>[2x]GAMAKVQVNNVVVLDNPSP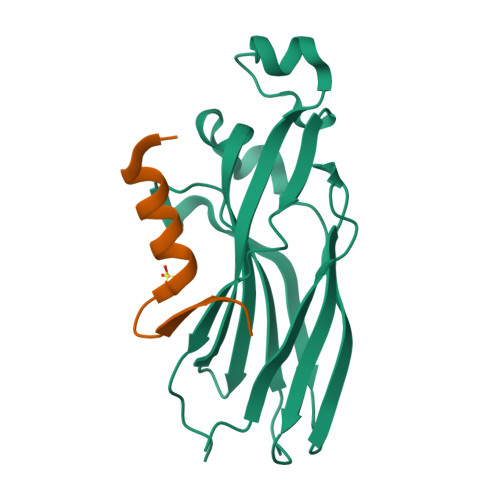FYNPFQFEITFECIEDLSEDLEWKIIYVGSAESEEYDQVLDSVLVGPVPAGRHMFVFQADAPNPGLIPDADAVGVTVVLITCTYRGQEFIRVGYYVNNEYTETELRENPPVKPDFSKLQRNILASNPRVTRFHINWEDN;>ASTERKWAELARRIRGAGGVTLNGFG[2x]>[4x]YAEGQRKRRNTIHEFKKSAKTTLIKIDPALKIKTKKVNTAD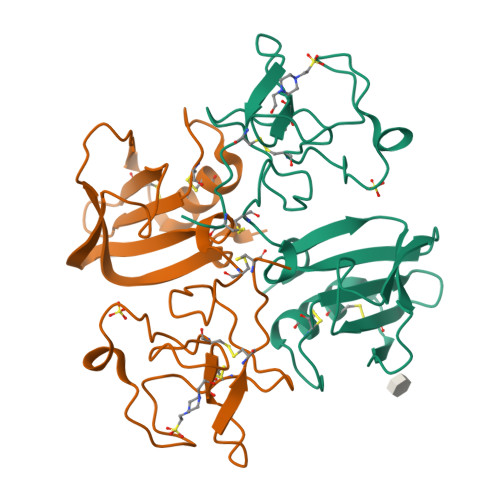QCANRCTRNKGLPFTCKAFVFDKARKQCLWFPFNSMSSGVKKEFGHEFDLYENKDYIRNCIIGEGESYKGTVSITKSGIKCQPWSSMIPHEHSFLPSSYRGKDLQENYCRNPRGEEGGPWCFTSNPEVRYEVCDIPQCSEVE>[2x]MTAVAQVVAKAEMLIRRPIAEVFEAFVDPAITARFWFSRGDARLEAGKRLRWHWDMYGVSQEIEVKDLQTNRRILIEWPNGDSNPSQVEWLFEELPGAGTFVSIRNSGFVGTP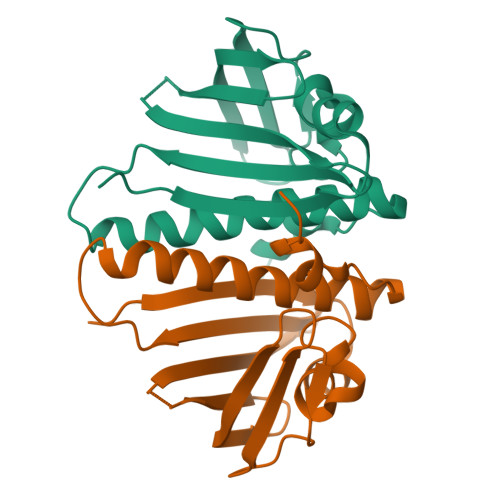EEVIPRVVDATEGFTLVLAGLKACLEHGIALNLVADRFPRGLDGLEHHHHHH> MSKFLDRFRYFKQKGETFADGHGQLLNTNRDWEDGYRQRWQHDKIVRSTHGVNCTGSCSWKIYVKNGLVTWETQQTDYPRTRPDLPNHEPRGCPSGASYSWYLYSANRLK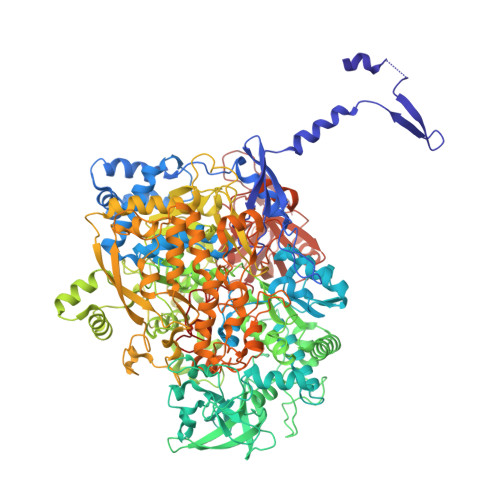YPMMRKRLMKMWREAKALHSDPVEAWASIIEDADKAKSFKQARGRGGFVRSSWQEVNELIAASNVYTIKNYGPDRVAGFSPIPAMSMVSYASGARYLSLIGGTCLSFYDWYCDLPPASPQTWGEQTDVPESADWYNSSYIIAWGSNVPQTRTPDAHFFTEVRYKGTKTVAVTPDYAEIAKLCDLWLAPKQGTDAAMALAMGHVMLREFHLDNPSQYFTDYVRRYTDMPMLVMLEERDGYYAAGRMLRAADLVDALGQENNPEWKTVAFNTNGEMVAPNGSIGFRWGEKGKWNLEQRDGKTGEETELQLSLLGSQDEIAEVGFPYFGGDGTEHFNKVELENVLLHKLPVKRLQLADGSTALVTTVYDLTLANYGLERGLNDVNCATSYDDVKAYTPAWAEQITGVSRSQIIRIAREFADNADKTHGRSMIIVGAGLNHWYHLDMNYRGLINMLIFCGCVGQSGGGWAHYVGQEKLRPQTGWQPLAFALDWQRPARHMNSTSYFYNHSSQWRYETVTAEELLSPMADKSRYTGHLIDFNVRAERMGWLPSAPQLGTNPLTIAGEAEKAGMNPVDYTVKSLKEGSIRFAAEQPENGKNHPRNLFIWRSNLLGSSGKGHEFMLKYLLGTEHGIQGKDLGQQGGVKPEEVDWQDNGLEGKLDLVVTLDFRLSSTCLYSDIILPTATWYEKDDMNTSDMHPFIHPLSAAVDPAWEAKSDWEIYKAIAKKFSEVCVGHLGKETDIVTLPIQHDSAAELAQPLDVKDWKKGECDLIPGKTAPHIMVVERDYPATYERFTSIGPLMEKIGNGGKGIAWNTQSEMDLLRKLNYTKAEGPAKGQPMLNTAIDAAEMILTLAPETNGQVAVKAWAALSEFTGRDHTHLALNKEDEKIRFRDIQAQPRKIISSPTWSGLEDEHVSYNAGYTNVHELIPWRTLSGRQQLYQDHQWMRDFGESLLVYRPPIDTRSVKEVIGQKSNGNQEKALNFLTPHQKWGIHSTYSDNLLMLTLGRGGPVVWLSEADAKDLGIADNDWIEVFNSNGALTARAVVSQRVPAGMTMMYHAQERIVNLPGSEITQQRGGIHNSVTRITPKPTHMIGGYAHLAYGFNYYGTVGSNRDEFVVVRKMKNIDWLDGEGNDQVQESVK> GAMGSAVSESQLKKMVSKYKYRDLTVRETVNVITLYKDLKPVLDSYGTGSRELMNLTGT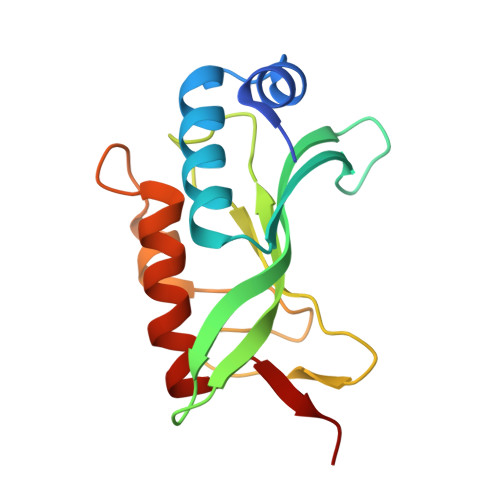IPVPYRGNTYNIPICLWLLDTYPYNPPICFVKPTSSMTIKTGKHVDANGKIYLPYLHEWKHPQSDLLGLIQVMIVVFGDEPPVFSRP>[2x]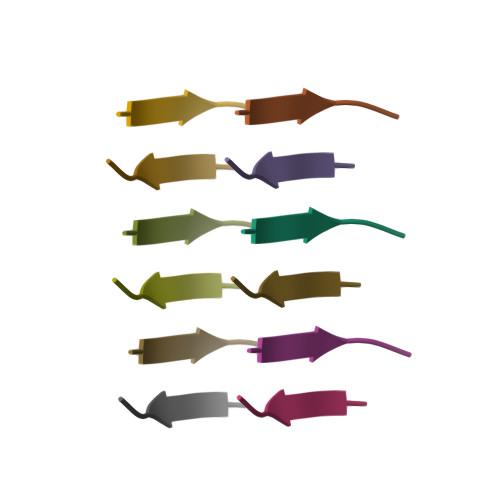MMHFGN> EWINVMNETKALMKEVMDIPEGYEILFFGGGASLQFLMVAMNLLNKKACYLDTGVWASKAIKEAENIGEVKIIGTSKDKNYTYIPEYQIPSDYDYFHITTNNTIYGTEIRKDIESPIPLVAD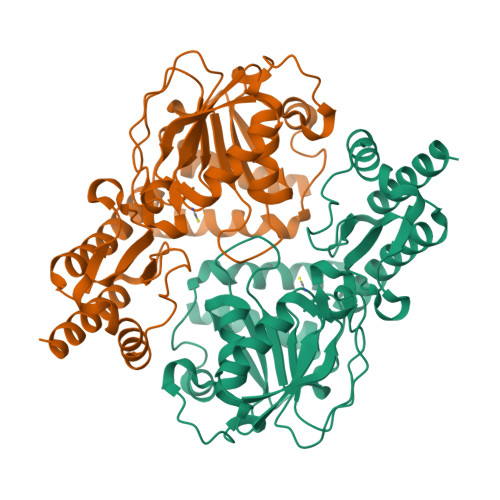MSSDILSKPIDISKYSLIYAGAQKNCGAAGVTIVIIKKEILGKVQRKIPIILDYQVHILNNSMYNTPPVISIFTVNQTLKYIKKIGGLKKIQELNEEKARLLYAEIDRNKIFRGTVRKKDRSIMNVCFVMEEQYKQLENEFSEYALQKGIIGIKGHRSVGGFRASIYNAVTIESVQALIKCMHDFEQLHTH2-oxo-3-(phosphonooxy)propanoic acid | C3 H5 O7 P | 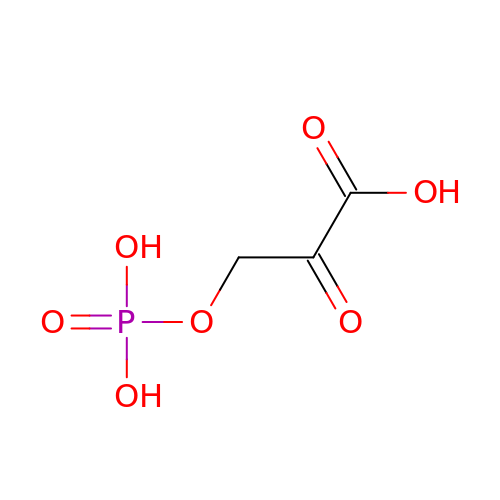LFLUCDOSQPJJBE-UHFFFAOYSA-N>GGGCCNGUCGUCUAXCCUGGUUAGGACGCCGCCCUUACAAGGCGGAGGXCCUGGGUUCGAGUCCCAGCGGGC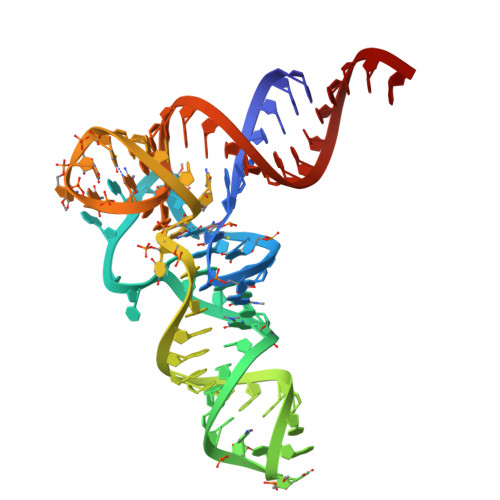CCACCA[2x]>[4x]MASSNVTLSNDEVLRLVKDWNFTWSVVFLLITIVLQYGYPSRSMFVYVIKMFVLWLLWPASMALSIFCAVYPIDLASQIISGILAATSCAMWISYFVQSIRLFMRTGSWWSFNP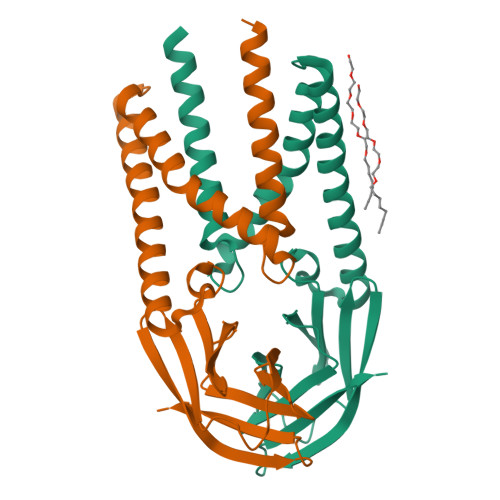ESNCLLNVPIGGTTVVRPLVEDSTSVTAVVTDGYLKMAGMHFGACDFQRLPSEVTVAKPNVLIALKMIKRQAYGTNSGVAIYHRYKAGNYRRPPIIQDQELALLRA> GEMKRAAIIIDDFGGDVKGVDDFLTGEIPVTVAVMP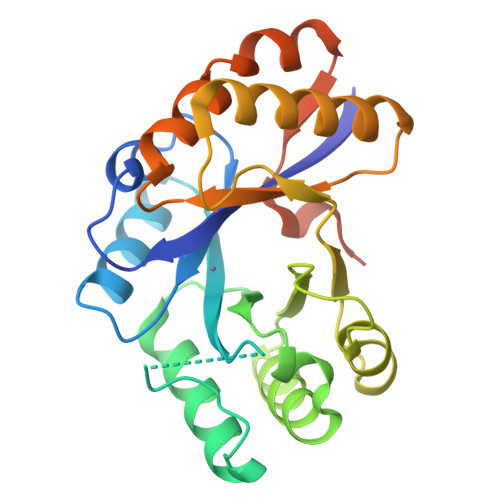FLEHSTKQAEIAQAAGLEVIVHMPLEPKKGKISWLGPSGITSNLSVGEVKSRVRKAFDDIPYAVGLNNHMGSKIVENEKIMRAILEVVKEKNAFIIDSGTSPHSLIPQLAEELEVPYATRSIFLDNTHSSRKEVIKNMRKLAKKAKQGSEPIGIGHVGVRGDETYAGIRSMLDEFQAESIQLVPVSQLLPSPIEEDHNKFWQQPFQAKE>[2x]MHHHHHHMET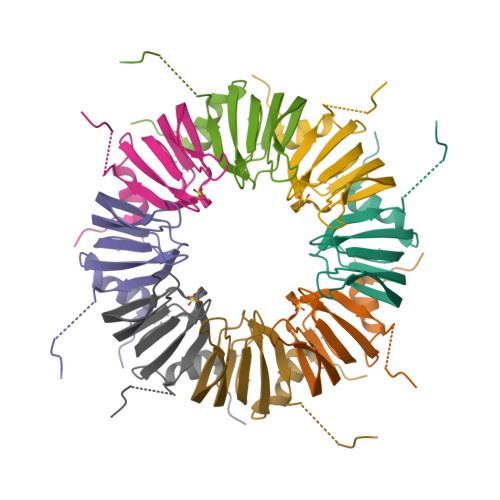PLDLLKLNLDERVYIKLRGARTLVGTLQAFDSHCNIVLSDAVETIYQLNNEELSESERRCEMVFIRGDTVTLISTPSEDDDGAVEI> MVKGSVHLWGKDGKASLISVDSIALVWFIKLCTSEEAKSMVAGLQIVFSNNTDLSSDGKLPVLILDNGTKVSGYVNIVQFLHKNICTSKYEKGTDYEEDLAIVRKKDRLLEYSLLNYVDVEISRLTDYQLFLNTKNYNEYTKKLFSKLLYFPMWYNTPLQLRSQARENCEEIIGSLTLEDDEEFVESKAMESASQLAQSKTFKIAHKNKIKGKQELQQVKYNLQFDNRLQSCVSNWLA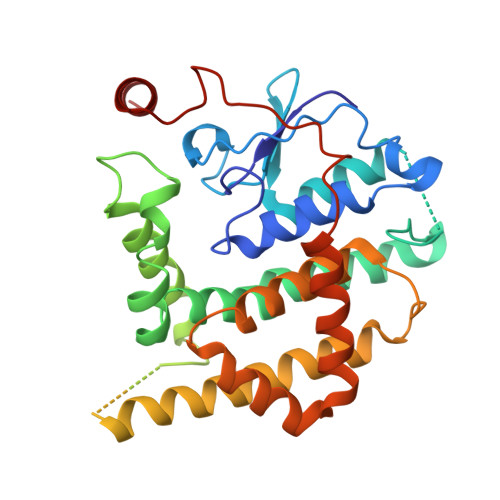ARKKLDDSVILSSDLLFLANLYVQLGLPDGNRIRSKLEQTFGSELLNSMSNKIDDFVHRPSNNLEQRDPQFREQGNVVMSLYNLACKYI> CGCGCA;> TGCGC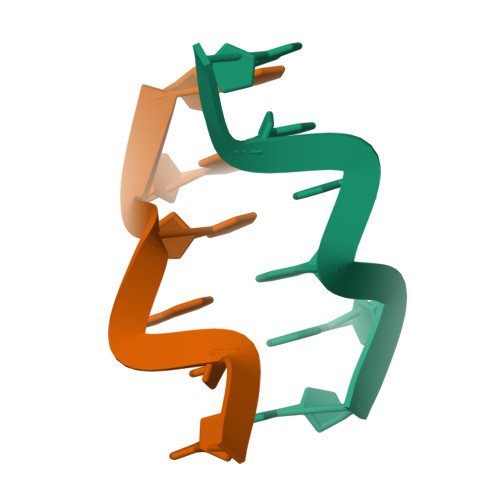G;>TG[2x]>[4x]MNITGKGAYDTGTYANLFQRSGYREDEIKARLEQTWNDLFYGDEHTRIYYPVGDDKGYMLDTGNDDVRSAGMSYGMMMAVQMDKKHEFDRLWNYAYTYMQHTEGRYKDYFAWHCKPDGTRLSPGPAPDGEEFFAMA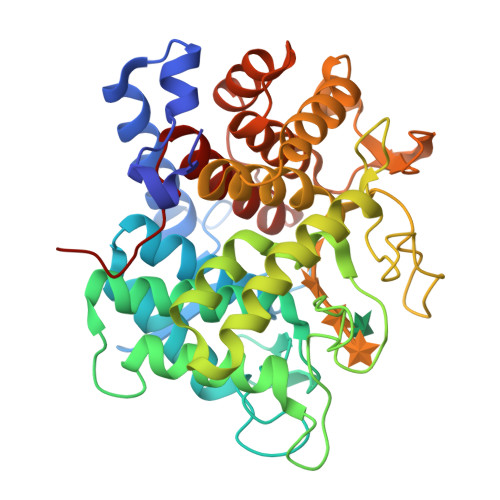LFFASNRWGDGPAPYDYQAQARKILHACLHQGEQGEGDPMWEPSNRLIKFIPELPFSDPSYHLPHFYELFAQYANEQDRTFWKEAAEASRAYLRTACHPVTGLSPEYANYDGTPAPVQLHGDFRHFYSDAYRVAANVALDWEWFRKDPWQVQQSNRIQAFFSDIDVSDYRRYTIEGEPFNEPALHPVGLLATNAMASLAADGPDADSFVKRFWNTPLRQGKRRYYDNCLYFFTMLALSGNYRVYQQAAA> 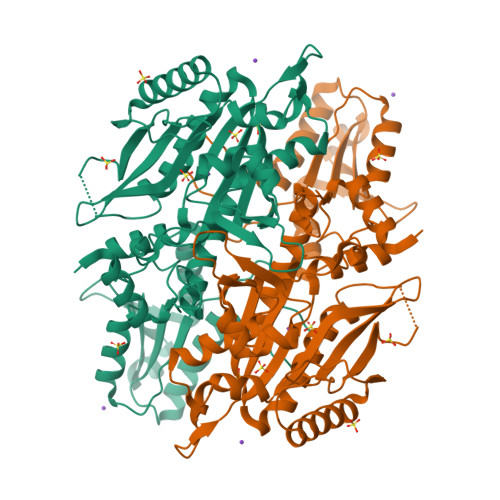MGSSHHHHHHSSGLVPRGSHMASATKNASSATPATMTSMVSQRQDLFMTDPLSPGSMFFLPNGAKIFNKLIEFMKLQQKFKFGFNEVVTPLIYKKTLWEKSGHWENYADDMFKVETTDEEKEEYGLKPMNCPGHCLIFGKKDRSYNELPLRFSDFSPLHRNEASGALSGLTRLRKFHQDDGHIFCTPSQVKSEIFNSLKLIDIVYNKIFPFVKGGSGAESNYFINFSTRPDHFIGDLKVWNHAEQVLKEILEESGKPWKLNPGDGAFYGPKLDIMVTDHLRKTHQVATIQLDFQLPERFDLKFKDQDNSYKRPIMIHRATFGSIERFMALLIDSNEGRWPFWLNPYQAVIIPVNTKNVQQLDMCTALQKKLRNELEADDMEPVPLNDWHFNVDLDIRNEPVGYRIKSAILKNYSYLIIVGDEEVQLQKYNIRERDNRKSFEKLTMSQIWEKFIELEKNYK> RETSEK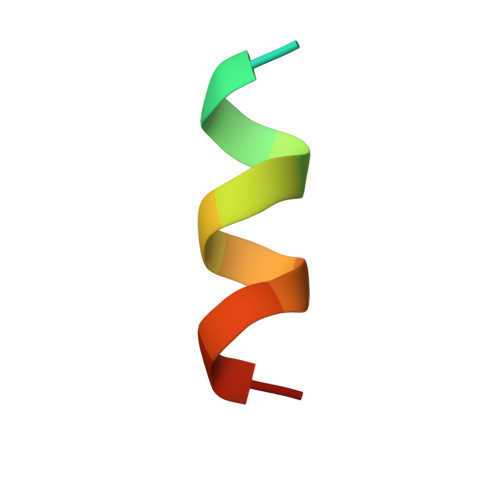FKLLFQSYN>[6x]GSHMGQGG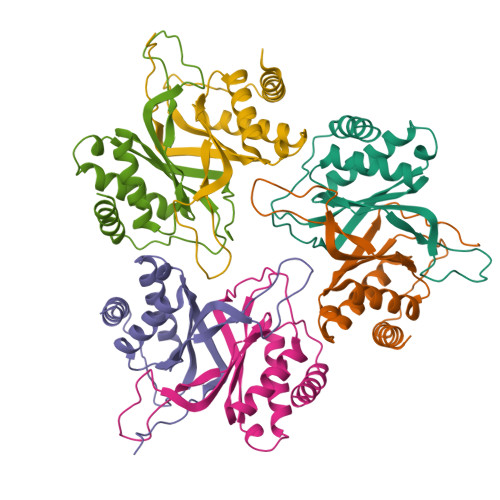SNPKFENIAEGLRALLARSHVERTTDEGTWVAGVFVYGGSKTSLYNLRRGTALAIPQCRLTPLSRLPFGMAPGPGPQPGPLRESIVCYFMVFLQTHIFAEVLKDAIKDLVMTKPAPTCNIRVTVCSFDDGVDLPPWFPPMVEGAAA>PLNSPNVYDVTAWRIKGQPKVTAESDIGAVINDIIADIKKRQSTPETRPGAVVIIPPGDYDLHTQVVVDVDYLTIAGFGHGFFSRSIKDNVDTTGWLNLQPGGSHIRVLTPPTSPQAFLVRRDGSPRLSGIVFKDFCLDGVSFVPDGNSYKNGKTGIDVASDNDSIHITGMGFVYLEHALIVRGADALRVHDNMVAECGNCVELTGAGQATIVSDNLMGAGPEGVTLLAENHEGLLVTGNNFFPRGRSLLEFTGCNRCSVTSNRFQGFYPGMMRLLNGCKENLITS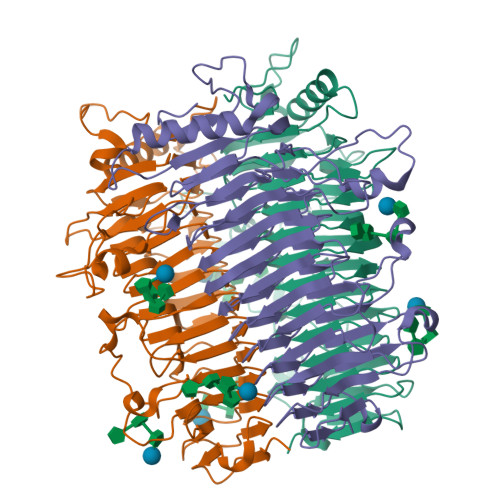NHFRRGTEGFPPFIDRTNGLDDLYGVIHAMGDNNLISNNLFAYDVPPGKIAPAGAQPTIMLIAGGDGNVIATNHVISNVDTQHVVLDGSATRSKVLDSGAASTITSYSPDTAIRPTPH[3x]> GGGGUUAUGUGUGCCCGGCAUGGGUGCAGUCUAUAGGGUGAGAGUCCCGAACUGUGAAGGCAGAAGUAACAGUUAGCCUAACGCAAGGGUGUCCGUGGCGACAUGGAAUCUGAAGGAAGCGGACGGCAAACCUUCGGUCUGAGGAACACGAACUUCAUAUGAGGCUAGGUAUCAAUGGAUGAGUUUGCAUAACAAAACAAAGUCCUUUCUGCCAAAGUUGGUACAGAGUAAAUGAAGCAGAUUGAUGAAGGGAAAGACUGCAUUCUUACCCGGGGAGGUCUGGAAACAGAAGUCA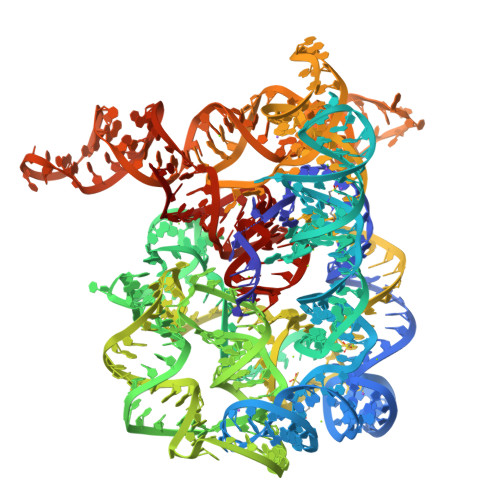GGAGAAGUCAUAGUACCCUGUUCGCAGGGGAAGGACGGAACAAGUAUGGCGUUCGCGCCUAAGCUUGAACGGCCGUAUACCGAACGGUACGUACGGUCGUGUG> DVPYVLVKTNMV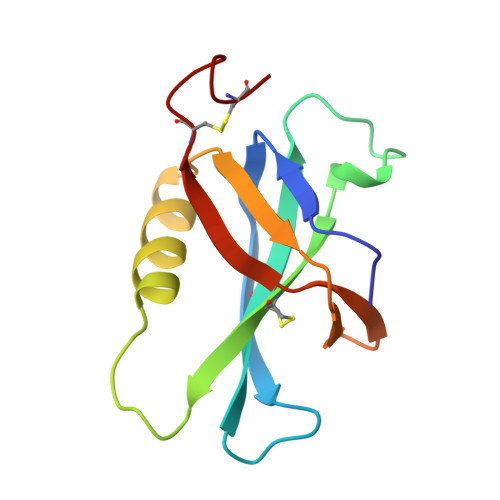VTSVAMKPYEVTPTRMLVCGIAAKLGAAASSPDAHVPFCFGKDLKRPGSSPMEVMLRAVFMQQRPLRMFLGPKQLTFEGKPALELIRMVECSGKQDCP2,2,2-tris(fluoranyl)-~{N}-[4-[3-[2-[[(3~{S})-piperidin-3-yl]amino]pyrimidin-4-yl]pyridin-2-yl]oxynaphthalen-1-yl]ethanesulfonamide 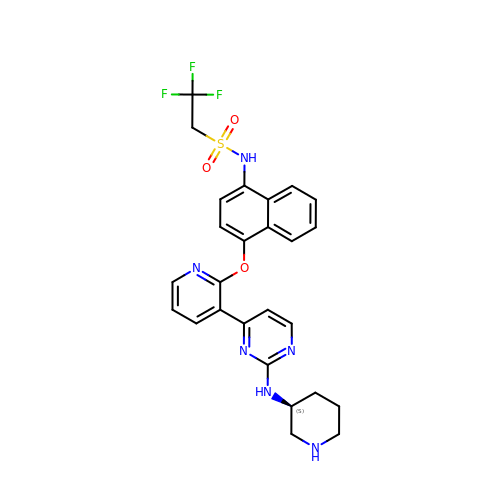| C26 H25 F3 N6 O3 S | LVBYPSVRFGNRPW-KRWDZBQOSA-N> MTVRKNQATLTADEKRRFVAAVLELKRSGRYDEFVRTHNEFIMSDTDSGERTGHRSPSFLPWHRRFLLDFEQALQSVDSSVTLPYWDWSADRTVRASLWAPDFLGGTGRSTDGRVMDGPFAASTGNWPINVRVDSRTYLRRSLGGSVAELPTRAEVESVLAISAYDLPPYNSASEGFRNHLEGWRGVNLHNRVHVWVGGQMATGVSPNDPVFWLHHAYVDKLWAEWQRRHPDSAYVPTGGTPDVVDLNETMKPWNTVRPADLLDHTAYYTFDALEHHHHHH;> MPEITRRRALTAAAAVAATASAAVTLAAPAASAAGHHEPAAPESFDEVYKGRRIQGRPAGGGAHHHEHGGGYEVFVDGVQLQVMRNADGSWISVVSHYDPVPTPRAAARAA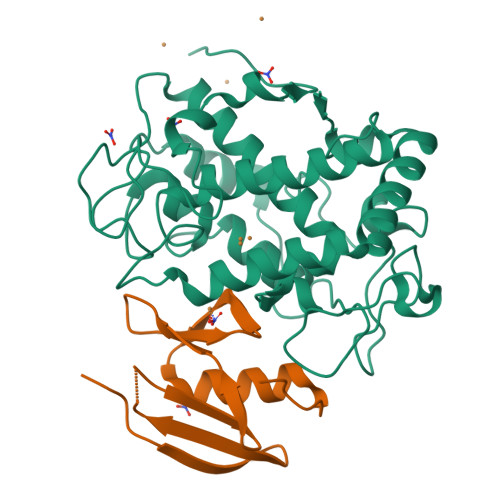VDELQGAPLLPFPANLEHHHHHH> KVTMNDFDYLKLLGKGTFGKVILVREKATGRYYAMKILRKEVIIAKDEVAHTVTESRVLQNTRHPFLTALKYAFQTHDRLCFVMEYANGGELFFHLSRERVFTEERARFYGAEIVSALEYLHSRDVVYRDIKLENLMLDKDGHIKITDFGLCKEGISDGATMKTFCGTPEYLAPEVLEDNDYGRAVDWWGLGVVMYEMMCGRLPFYNQDHERLFELILMEEIRFPRTLSPEAKSLLAGLLKKDPKQRLGGGPSDAKEVMEHRFFLSINWQDVVQKKLLPPFKPQVT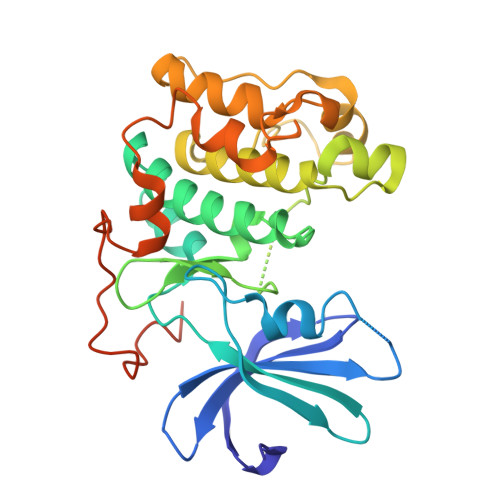SEVDTRYFDDEFTAQSITITPPDRYDSLG> GHIKQLLKNKRFEVIKALVESKKIKQEWLEDLYSILLKQDTDVEITQAKYEIIKLLLTEKKYLNFELLTKTLNLDQQTAIEIMRNPFKEVYFPTYNIENPEESRLNKALIIPLSNQTFTLNTFVNSQDLETIKEATNKNFFVIFDNIFSGKSYQLAVAAGLIAKEKEILDNVAFTGEVSSNGFIIPVNHLEEKKEITEKAKKVLITPEDIENLEELSFWLNPEHLPVIFIHINKPELALQSL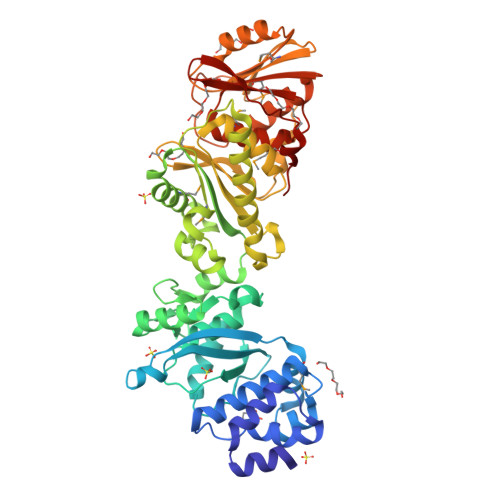KQMEDAIKKDERFKYFKLENLKKFYRLEDQDMYLITPSVDFSNREELIKILNEFREKVSKLLTLEGVIKDHNKVVLNISAGISTLALYFGVILGNRQASIIYHYQKEYHKVIDLTDNPRKIKEKKSEFEKISVNKNIQDPLMIIIYLASHNPIEKGLELKEKLRAKGELIIQSKEHQGNLEIGDWSDIVSEIYTAIDDNKQKENYMVFSAPVAIMLALGMALGYFLPIKVFHYNRDEYIEVPIKLNEEILRSPF> MAGNQRQGVAFIRVNGMELESMEGASFTPSGITREEVTGSRVYGWKGKPRAAKVECKIPGGGPIGLDEIIDWENITVEFQADTGETWMLANAWQA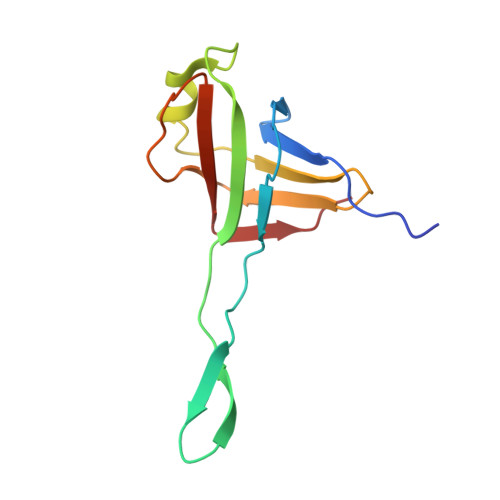DEPKNDGGEISLVLMAKQSKRIA>[2x]MARAAFLFKTVGFGGLQNVPINDELSSHLLRAGNSPWQLTQFLDWISLGRGLATSALVPTAGSRYYQMSCLLSGTLQIPFRPNHRWGDIRFLRLVWSAPTLDGLVVAPPQVLAQPALQAQADRVYDCDDYPFLARDPRFKHRVYQQLSAVTLLNLTGFGPISYVRVDEDMWSGDVNQLLMNYFGHTFAEIAYTLCQASANRPWEYDGTYARMTQIVLSLFWLSYVGVIHQQNTYRTFYFQCNRRGDAAEVWILSCSLNHSAQIRPGNRSLFVMPTSPDWNMDVNLILSSTLTGCLCSGSQLPLIDNNSVPAVSRNIHGWTGRAGNQLHGFQVRRMVTEFCDRLRRDGVMTQAQQNQVEALADQTQQFKRDKLETWAREDDQYNQAHPNSTMFRTKPFTNAQWGRGNTGATSAAIAALI;>[6x]MGNASSIVQTINVTGDGNVFKPSAETSSTAVPSLSLSPGMLNPGGVPWIAVGDETSVTSPGALRRMTSKDIPETAIINTDNSSGAVPSESALVPYIDEPLVVVTEHAITNFTKAEMALEFNREFLDKMRVLSVSPKYSDLLTYVDCYVGVSARQALNNFQKQVPVITPTRQTMYVDSIQAALKALEKWEIDLRVAQTLLPTNVPIGEVSCPMQSVVKLLDDQLPDDSLIRRYPKEAAVALAKRNGGIQWMDVSEGTVMNEAVNAVAASALAPSASAPPLEEKSKLTEQAMDLVTAAEPEIIASLAPVPAPVFAIPPKPADYNVRTLRIDEATWLRMIPKSMNTPFQIQVTDNTGTNWHLNLRGGTRVVNLDQIAPMRFVLDLGGKSYKETSWDPNGKKVGFIVFQSKIPFELWTAASQIGQATVVNYVQLYAEDSSFTAQSIIATTSLAYNYEPEQLNKTDPEMNYYLLATFIDSAAITPTNMTQPDVWDALLTMSPLSAGEVTVKGAVVSEVVPADLIGSYTPESLNASLPNDAARCMIDRASKIAEAIKIDDDAGPDEYSPNSVPIQGQLAISQLETGYGVRIFNPKGILSKIASRAMQAFIGDPSTIITQAAPVLSDKNNWIALAQGVKTSLRTKSLSAGVKTAVSKLSSSESIQNWTQGFLDKVSAHFPAPKPDCPTSGDSGESSNRRVKRDSYAGVVKRGYTR;>[3x]MEVCLPNGHQVVDLINNAFEGRVSIYSAQEGWDKTISAQPDMMVCGGAVVCMHCLGVVGSLQRKLKHLPHHRCNQQIRHQDYVDVQFADRVTAHWKRGMLSFVAQMHEMMNDVSPDDLDRVRTEGGSLVELNWLQVDPNSMFRSIHSSWTDPLQVVDDLDTKLDQYWTALNLMIDSSDLIPNFMMRDPSHAFNGVKLGGDARQTQFSRTFDSRSSLEWGVMVYDYSELEHDPSKGRAYRKELVTPARDFGHFGLSHYSRATTPILGKMPAVFSGMLTGNCKMYPFIKGTAKLKTVRKLVEAVNHAWGVEKIRYALGPGGMTGWYNRTMQQAPIVLTPAALTMFPDTIKFGDLNYPVMIGDPMILG;> MANVWGVRLADSLSSPTIETRTRQYTLHDLCSDLDANPGREPWKPLRNQRTNNIVAVQLFRPLQGLVLDTQLYGFPGAFDDWERFMREKLRVLKYEVLRIYPISNYSNEHVNVFVANALVGAFLSNQAFYDLLPLLIINDTMIGDLLGTGASLSQFFQSHGDVLEVAAGRKYLQMENYSNDDDDPPLFAKDLSDYAKAFYSDTYEVLDRFFWTHDSSAGVLVHYDKPTNGHHYLLGTLTQMVSAPPYIINATDAMLLESCLEQFSANVRARPAQPVTRLDQCYHLRWGAQYVGEDSLTYRLGVLSLLATNGYQLARPIPRQLTNRWLSSFVSQIMSDGVNETPLWPQERYVQIAYDSPSVVDGATQYGYVRKNQLRLGMRISALQSLSDTPSPVQWLPQYTIDQAAMDEGDLMVSRLTQLPLRPDYGNIWVGDALSYYVDYNRSHRVVLSSELPQLPDTYFDGDEQYGRSLFSLARKIGDRSLVKDTAVLKHAYQAIDPNTGKEYLRSRQSVAYFGASAGHSGADQPLVIEPWIQGKISGVPPPSSVRQFGYDVARGAIVDLARPFPSGDYQFVYSDVDQVVDGHDDLSISSGLVESLLSSCMHATAPGGSFVVKINFPTRPVWHYIEQKILPNITSYMLIKPFVTNNVELFFVAFGVHQHSSLTWTSGVYFFLVDHFYRYETLSTISRQLPSFGYVDDGSSVTGIETISIENPGFSNMTQAARIGISGLCANVGNARKSIAIYESHGARVLTITSRRSPASARRKSRLRYLPLIDPRSLEVQARTILPADPVLFENVSGASPHVCLTMMYNFEVSSAVYDGDVVLDLGTGPEAKILELIPATSPVTCVDIRPTAQPSGCWNVRTTFLELDYLSDGWITGVRGDIVTCMLSLGAAAAGKSMTFDAAFQQLIKVLSKSTANVVLVQVNCPTDVVRSIKGYLEIDSTNKRYRFPKFGRDEPYSDMDALEKICRTAWPNCSITWVPLSYDLRWTRLALLESTTLSSASIRIAELMYKYMPIMRIDIHGLPMEKRGNFIVGQNCSLVIPGFNAQDVFNCYFNSALAFSTEDVNAAMIPQVSAQFDATKGEWTLDMVFSDAGIYTMQALVGSNANPVSLGSFVVDSPDVDITDAWPAQLDFTIAGTDVDITVNPYYRLMTFVRIDGQWQIANPDKFQFFSSASGTLVMNVKLDIADKYLLYYIRDVQSRDVGFYIQHPLQLLNTITLPTNEDLFLSAPDMREWAVKESGNTICILNSQGFVLPQDWDVLTDTISWSPSIPTYIVPPGDYTLTPL;>MKRIPRKTKGKSSGKGNDSTERADDGSSQLRDKQNNKAGPATTEPGTSNREQYKARPGIASVQRATESAEMPMKNNDEGTPDKKGNTKGDLVNEHSEAKDEADEATKKQAKDTDKSKAQVTYSDTGINNANELSRSGNVDNEGGSNQKPMSTRIAEATSAIVSKHPARVGLPPTASSGHGYQCHVCSAVLFSPLDLDAHVASHGLHGNMTLTSSDIQRHITEFISSWQNHPIVQVSADVENKKTAQLLHADTPRLVTWDAGLCTSFKIVPIVPAQVPQDVLAYTFFTSSYAIQSPFPEAAVSRIVVHTRWASNVDFDRDSSVIMAPPTENNIHLFKQLLNTETLSVRGANPLMFRANVLHMLLEFVLDNLYLNRHTGFSQDHTPFTEGANLRSLPGPDAEKWYSIMYPTRMGTPNVSKICNFVASCVRNRVGRFDRAQMMNGAMSEWVDVFETSDALTVSIRGRWMARLARMNINPTEIEWALTECAQGYVTVTSPYAPSVNRLMPYRISNAERQISQIIRIMNIGNNATVIQPVLQDISVLLQRISPLQIDPTIISNTMSTVSESTTQTLSPASSILGKLRPSNSDFSSFRVALAGWLYNGVVTTVIDDSSYPKDGGSVTSLENLWDFFILALALPLTTDPCAPVKAFMTLANMMVGFETIPMDNQIYTQSRRASAFSTPHTWPRCFMNIQLISPIDAPILRQWAEIIHRYWPNPSQIRYGAPNVFGSANLFTPPEVLLLPIDHQPANVTTPTLDFTNELTNWRARVCELMKNLVDNQRYQPGWTQSLVSSMRGTLDKLKLIKSMTPMYLQQLAPVELAVIAPMLPFPPFQVPYVRLDRDRVPTMVGVTRQSRDTITQPALSLSTTNTTVGVPLALDARAITVALLSGKYPPDLVTNVWYADAIYPMYADTEVFSNLQRDMITCEAVQTLVTLVAQISETQYPVDRYLDWIPSLRASAATAATFAEWVNTSMKTAFDLSDMLLEPLLSGDPRMTQLAIQYQQYNGRTFNIIPEMPGSVIADCVQLTAEVFNHEYNLFGIARGDIIIGRVQSTHLWSPLAPPPDLVFDRDTPGVHIFGRDCRISFGMNGAAPMIRDETGLMVPFEGNWIFPLALWQMNTRYFNQQFDAWIKTGELRIRIEMGAYPYMLHYYDPRQYANAWNLTSAWLEEITPTSIPSVPFMVPISSDHDISSAPAVQYIISTEYNDRSLFCTNSSSPQTIAGPDKHIPVERYNILTNPDAPPTQIQLPEVVDLYNVVTRYAYETPPITAVVMGVP[15x];> MAYIAVPAVVDSRSSEAIGLLESFGVDAGADANDVSYQDHDYVLDQLQYMLDGYEAGDVIDALVHKNWLHHSVYCLLPPKSQLLEYWKSNPSAIPDNVDRRLRKRLMLKKDLRKDDEYNQLARAFKISDVYAPLISSTTSPMTMIQNLNQGEIVYTTTDRVIGARILLYAPRKYYASTLSFTMTKCIIPFGKEVGRVPHSRFNVGTFPSIATPKCFVMSGVDIESIPNEFIKLFYQRVKSVHANILNDISPQIVSDMINRKRLRVHTPSDRRAAQLMHLPYHVKRGASHVDVYKVDVVDMLFEVVDVADGLRNVSRKLTMHTVPVCILEMLGIEIADYCIRQEDGMLTDWFLLLTMLSDGLTDRRTHCQYLINPSSVPPDVILNISITGFINRHTIDVMPDIYDFVKPIGAVLPKGSFKSTIMRVLDSISILGIQIMPRAHVVDSDEVGEQMEPTFEQAVMEIYKGIAGVDSLDDLIKWVLNSDLIPHDDRLGQLFQAFLPLAKDLLAPMARKFYDNSMSEGRLLTFAHADSELLNANYFGHLLRLKIPYITEVNLMIRKNREGGELFQLVLSYLYKMYATSAQPKWFGSLLRLLICPWLHMEKLIGEADPASTSAEIGWHIPREQLMQDGWCGCEDGFIPYVSIRAPRLVIEELMEKNWGQYHAQVIVTDQLVVGEPRRVSAKAVIKGNHLPVKLVSRFACFTLTAKYEMRLSCGHSTGRGAAYSARLAFRSDLA;> MSSMILTQFGPFIESISGITDQSNDVFEDAAKAFSMFTRSDVYKALDEIPFSDDAMLPIPPTIYTKPSHDSYYYIDALNRVRRKTYQGPDDVYVPNCSIVELLEPHETLTSYGRLSEAIENRAKDGDSQARIATTYGRIAESQARQIKAPLEKFVLALLVAEAGGSLYDPVLQKYDEIPDLSHNCPLWCFREICRHISGPLPDRAPYLYLSAGVFWLMSPRMTSAIPPLLSDLVNLAILQQTAGLDPSLVKLGVQICLHAAASSSYAWFILKTKSIFPQNTLHSMYESLEGGYCPNLEWLEPRSDYKFMYMGVMPLSAKYARSAPSNDKKARELGEKYGLSSVVGELRKRTKTYVKHDFASVRYIRDAMACTSGIFLVRTPTETVLQEYTQSPEIKVPIPQKDWTGPIGEIRILKDTTSSIARYLYRTWYLAAARMAAQPRTWDPLFQAIMRSQYVTARGGSGAALRESLYAINVSLPDFKGLPVKAATKIFQAAQLANLPFSHTSVAILADTSMGLRNQVQRRPRSIMPLNVPQQQVSAPHTLTADYINYHMNLSTTSGSAVIEKVIPLGVYASSPPNQSINIDISACDASITWDFFLSVIMAAIHEGVASSSIGKPFMGVPASIVNDESVVGVRAARPISGMQNMIQHLSKLYKRGFSYRVNDSFSPGNDFTHMTTTFPSGSTATSTEHTANNSTMMETFLTVWGPEHTDDPDVLRLMKSLTIQRNYVCQGDDGLMIIDGTTAGKVNSETIQKMLELISKYGEEFGWKYDIAYDGTAEYLKLYFIFGCRIPNLSRHPIVGKERANSSAEEPWPAILDQIMGVFFNGVHDGLQWQRWIRYSWALCCAFSRQRTMIGESVGYLQYPMWSFVYWGLPLVKAFGSDPWIFSWYMPTGDLGMYSWISLIRPLMTRWMVANGYVTDRCSPVFGNADYRRCFNELKLYQGYYMAQLPRNPKKSGRAAPREVREQFTQALSDYLMQNPELKSRVLRGRSEWEKYGAGIIHNPPSLFDVPHKWYQGAQEAAIATREELAEMDETLMRARRHSYSSFSKLLEAYLLVKWRMCEAREPSVDLRLPLCAGIDPLNSDPFLKMVSVGPMLQSTRKYFAQTLFMAKTVSGLDVNAIDSALLRLRTLGADKKALTAQLLMVGLQESEADALAGKIMLQDVNTVQLARVVNLAVPDTWMSLDFDSMFKHHVKLLPKDGRHLNTDIPPRMGWLRAILRFLGAGMVMTATGVAVDIYLEDIHGGGRSLGQRFMTWMRQEGRSA

MRV is a prototypical member of the Reoviridae family of segmented double-stranded RNA (dsRNA) viruses, which is further divided into two subfamilies based on the presence or absence of turrets on the inner capsids: turreted (Spinareovirinae, including MRV) and nonturreted (Sedoreovirinae, including bluetongue virus (BTV) and the life-threatening rotavirus). MRV capsids are composed of two concentric protein layers, encapsulating 10 dsRNA segments. The outer layer of MRV consists of the protection protein σ3, membrane penetration protein μ1, and spike protein σ1. The inner layer consists of proteins λ1, σ2, and turret protein λ223.

The transcription enzyme complex (TEC) is comprised of λ3 and μ2 and is attached inside the inner layer. Asymmetric sub-particle reconstruction yielded near-atomic resolution (up to 3.0 Å) structures for five types of viral particles, all with visible side chain densities for atomic model building: from 6 h post-infection, core, virion, empty core, and empty virion were reconstructed; and for 48 h post-infection, structures of virion, empty virion, and outer shell particle were obtained. Inside the particle, reconstructions of virion and core particles clearly show that the layered RNA genome and densities of TEC (at red arrows) are underneath the inner shell, indicating that genome replication from ssRNA to dsRNA has been completed in the core. However, an asymmetric reconstruction of the TEC was obtained after focused classification in virions only, not in the empty virion. This result suggests that the RNA genome is important for stable docking of TEC to the inner layer protein shell, though it is not required for TEC incorporation into the capsid, as also suggested by the tomograms. The λ2 pentameric turret changes conformation during virus assembly: in the core, the turret is open, with a central channel 75 Å in diameter; in the virion, it closes, sealing off the channel. As the proteins μ1/σ3 coat the core to form the outer layer of the virion, the last two of the three Ig-like domains, acting as a rigid body, flip down 46° to close the channel, which is then sealed by σ1 attachment. Studies have shown that assembled core particles in the condensates are active in mRNA transcription, but this activity is inhibited after outer layer proteins μ1/σ3 and σ1 are incorporated to form virion particles. Our structural data align with these functional findings: in the core, the open conformation of the turret maximally facilitates mRNA export efficiency, while in the virion, the closed conformation of the turret suppresses transcription, leading to a virion in the quiescent state. The coating of outer layer proteins μ1, σ3, and σ1 occurs continuously throughout capsid formation and completes the virion particles, which eventually egress from the cell.(4R,5S)-3-(1-(4,5-dihydrothiazol-2-yl)azetidin-3-ylthio)-5-((2S,3R)-3-hydroxy-1-oxobutan-2-yl)-4-methyl-4,5- dihydro-1H-pyrrole-2-carboxylic 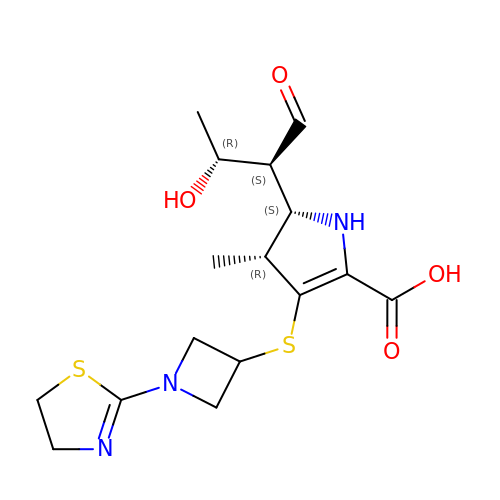acid | C16 H23 N3 O4 S2 | PGCJBZBFZXWIGF-CNVPUSNMSA-N> MPNNESIVVEIVKLKNFHVYRGV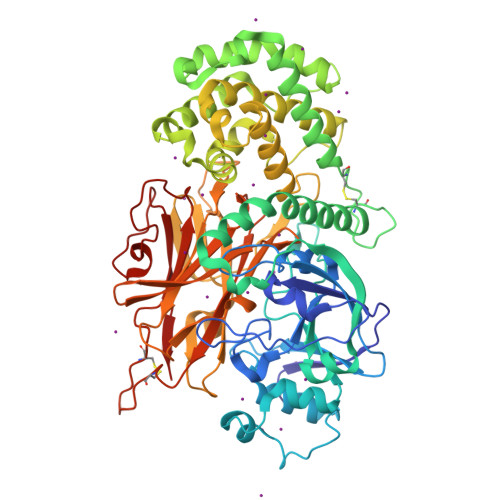SPIGVKDYQVGQKIVKSTSTDEHGNPVGLGNYDPHWQGLYAAEHLHHAASYAVDNNSGVPGGLFKIKLPEDVRFVRYENKDAAQAITPGRLYRALREEGLIKLTTAKELNETHFNSNQNFLTNELGKEKIILIDTDEFESFTDINGMKIPRLEFIIPWNIATEQVQVSEEVKVWYKGRDFSSLNAKERLELMMKLRGPYENDLTSYEAKFKDLIICRSASYYSSGSSCLDWEKIKTESQRIVKQIIEEHPELQSHSKNAVTDKEKLQKIYNDYAPKIDKLSSLKEGVSRATTALNIASWAAGLAETFSNKNADGLDKAAAVTAIIPGLGQAVGIANGIEKHDGEAIAINSIALSALVVAQAIPIVGEIADVVGAGLILAGGLAQLIQSVSPDTPPHVEPPHFYPQTSNHVTVGWLNQKIDEMIHAWYPHEGYRSHHFVIKIANDAPENTTMPITEIMAKLGSQTKQLDLVPERVWVYQNNNVITCTKQTVSLKTDRFAVIRPLFPTMLTKSRPIVVRMAYITGENSCTTDANPTCFPENPAIAVRVTPLPSNNECEWDHTPLHPSYQNGDKADFVRLGYRIGV galactinol | C12 H22 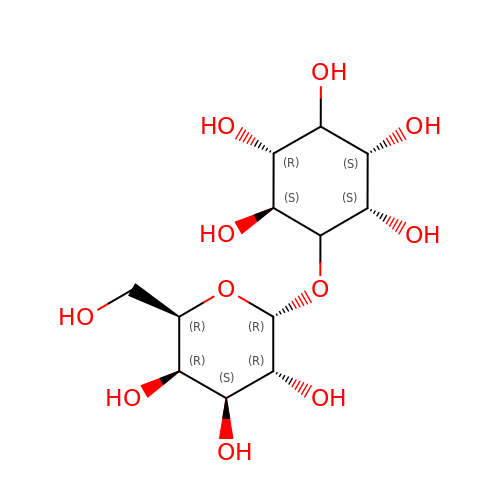O11 | VCWMRQDBPZKXKG-DXNLKLAMSA-N> MSVIVYRNNQSTLTLNGYTFQHLYQGAALVLTPVNAKTARTNSINGGVSISGRVDGGVHTLAIMVQKHSPDDKFLNDAKNSQEPVVF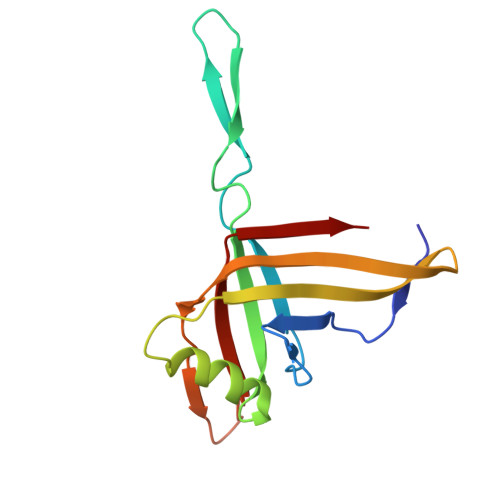DGSMKRAYTESGTLKKATTTLETGSITTQPTKTDNNQDPDDSRTYVIEFRNSVETF>[12x]SMSQSGEDLHSPTYLSWRKLQLSRAKLKASS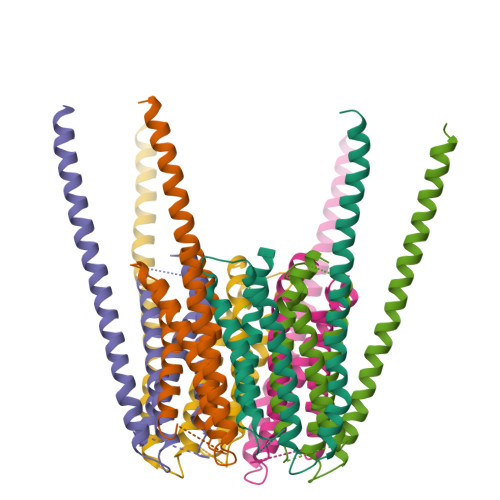KTSALLSGFAMVAMVEVQLDHDTNVPPGMLIAFAICTTLLVAVHMLALMISTCILPNIETVSNLHSISLVHESPHERLHWYIETAWAFSTLLGLILFLLEIAILCWVKFYDLSPPAAWSATVVLILVMIIFMAFAIHFYRSLVSHKYEVTVSGIRELEMLKEQMEQDHLEHHNNIRNNG> MTYRVKIHKQVVKALQSLPKAHYRRFLEFRDILEYEPVPREKFDVIKLEGTGDLDLYRARLGDYRVIYSVNWKDKVIKILKLKPRG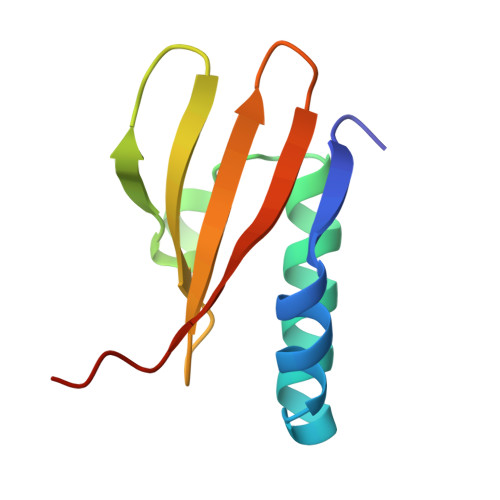RAYK> MLNFGKKPAYTTSNGSMYIGDSLELLESFPEESISLVMTSPPFALQRKKEYGNLEQHEYVDWFLSFAKVVNKKLKPDGSFVVDFGGAYMKGVPARSIYNFRVLIRMIDEVGFFLAEDFYWFNPSKLPSPIEWVNKRKIRVKDAVNTVWWFSKTEWPKSDITKVLAPYSDRMKKLIEDPDKFYTP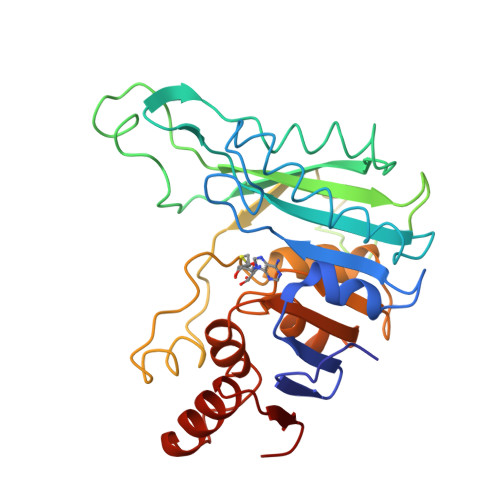KTRPSGHDIGKSFSKDNGGSIPPNLLQISNSESNGQYLANCKLMGIKAHPARFPAKLPEFFIRMLTEPDDLVVDIFGGSNTTGLVAERESRKWISFEMKPEYVAASAFRFLDNNISEEKITDIYNRILNGESLDLNSII> GAMDPRTITMHKDSTGHVGFIFKNGKITSIV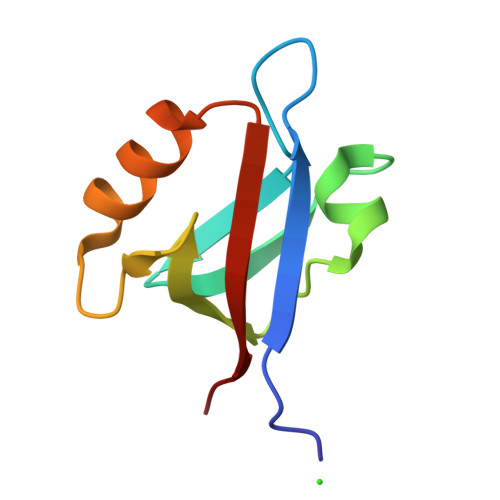KDSSAARNGLLTEHNICEINGQNVIGLKDSQIADILSTSGTVVTITIMPAF>MSEMDYLENATVIDESALTPEQRLGLKQAEERLERDHIFRLEKRSPEYTNCRYLCKLCLIHIENIQGAHKHIKEKRHKKNILEKQEESELRSLPPPSPAHLAALSVAVIELAKEHGITDDDLRVRQEIVEEMSKVITTFLPECSLRLYGSSLTRFALKSSDVNIDIKFPPKMNHPDLLIKVLGILKKNVLYVDVESDFHAKVPVVVCRDRKSGLLCRVSAGNDMACLTTDLLTALGKIEPVFIPLVLAFRYWAKLCYIDSQTDGGIPSYCFALMVMFFLQQRKPPLLPCLLGSWIEGFDPKRMDDFQLKGIVEEKFVKWECNSSSATKEKHGKSPL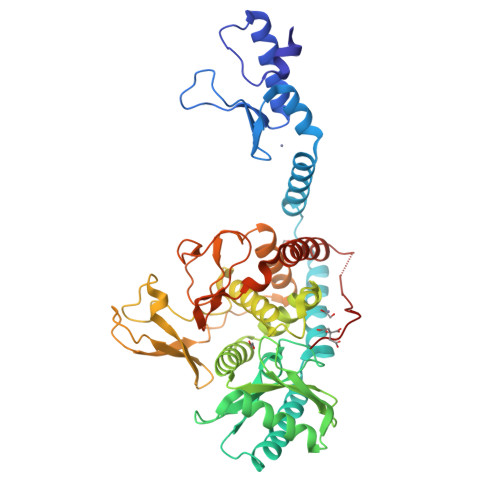ALETPNRVSLGQLWLELLKFYTLDFALEEYVICVRIQDILTRENKNWPKRRIAIEDPFSVKRNVARSLNSQLVYEYVVERFRAAYRYFACPQTKGGNKSTVDFKLEHHHHHH[2x]>GKINDWEEPRLDIEGFVVDYFTHRIRQNGMEWFGAPGLPSGVQPEHEMMRVMGTIFEKKHAENFETFSEQLLAVPRISFSLYQDVVRTVGNAQTDQSPMSYGRLIGLISFGGFVAAKMMESVELQGQVRNLFVYTS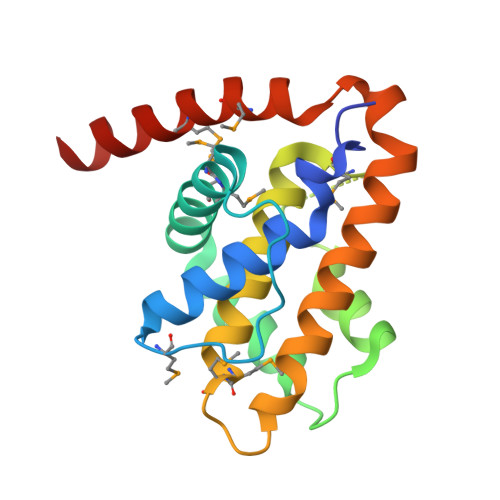LFIKTRIRNNWKEHNRSWDDFMTLGKQMKEDYERAEAEK[2x]>MSDLAAVDDWSTLRRIAIDAVSTGRN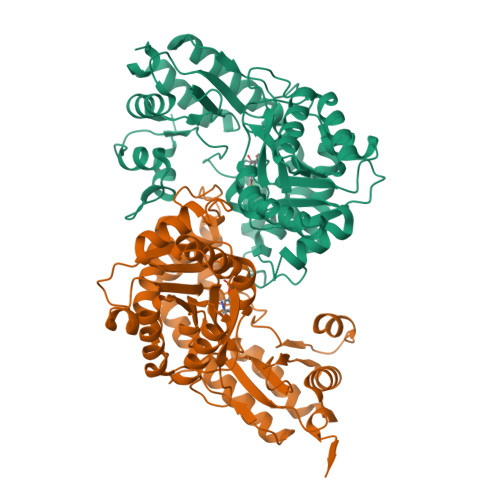PELKWLADHPEGTPAYALHLADPLEGAPEGLRQCLREAWDEPLDSYVLSHHGLPELRQAMERWFADDENWPRRRRLLTTATMTGTGPAMYDLLRTIKAREPEGPMAALVPRPGWDYRLFAHDVGYEPIGYHVPFTSPTGPEPGDLDRAVEQTRAKGLRPTVLVLNPQHYATGGNWTPEFVRYALSLADTLGMWVLVDNAYHGMTAAGTQPTSTVRLALDGGFEERLIHVRTLGKQFACNGWAVGSVTAMPDVIDEFAHRWRGFREYPGHAREQAAFAGWLNNPESRKWADERREAIRSNGDALLDALAEVSNTTRHCHGGSPFVLFEVPGGWSQEDFRQRLFADTGVLLASAQIPYAPDWVKVFLGRRPDRFLPAVEALRTRPSRAWQPRLEHHHHHHHH[4x]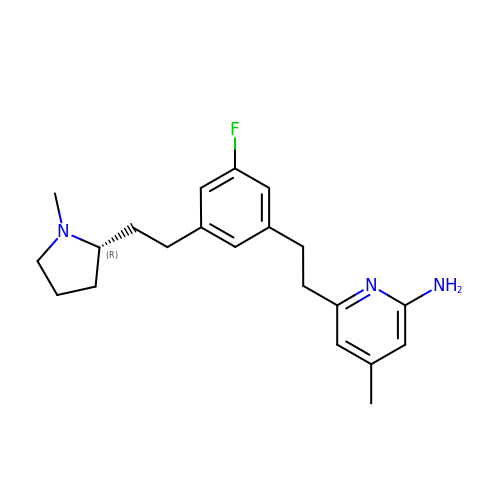6-[2-(3-fluoro-5-{2-[(2R)-1-methylpyrrolidin-2-yl]ethyl}phenyl)ethyl]-4-methylpyridin-2-amine | C21 H28 F N3 | LLEZATCTDGWSJC-FQEVSTJZSA-N>MIWKRKITLEALNAMGEGNMVGFLDIRFEHIGDDTLEATMPVDSRTKQPFGLLHG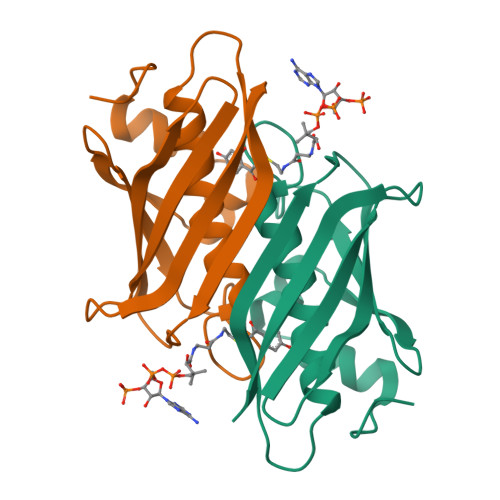GASVVLAESIGSVAGYLCTEGEQKVVGLEINANHVRSAREGRVRGVCKPLHLGSRHQVWQIEIFDEKGRLCCSSRLTTAIL[4x]> MGSDRSCVLSVFQTILKLVIFVAIFGAAISSRLFAVIKFESIIHEFDPWFNYRA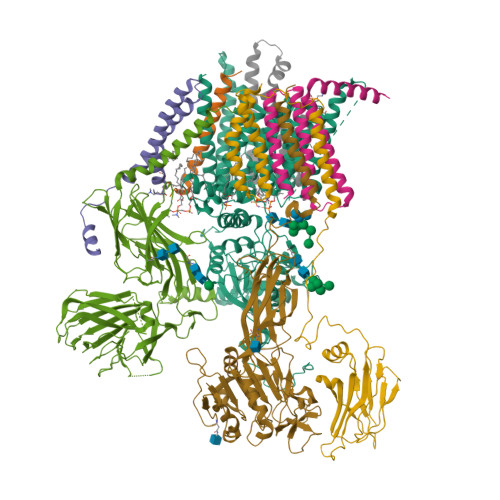TKYLVNNSFYKFLNWFDDRTWYPLGRVTGGTLYPGLMTTSAFIWHALRNWLGLPIDIRNVCVLFAPLFSGVTAWATYEFTKEIKDASAGLLAAGFIAIVPGYISRSVAGSYDNEAIAITLLMVTFMFWIKAQKTGSIMHATCAALFYFYMVSAWGGYVFITNLIPLHVFLLILMGRYSSKLYSAYTTWYAIGTVASMQIPFVGFLPIRSNDHMAALGVFGLIQIVAFGDFVKGQISTAKFKVIMMVSLFLILVLGVVGLSALTYMGLIAPWTGRFYSLWDTNYAKIHIPIIASVSEHQPVSWPAFFFDTHFLIWLFPAGVFLLFLDLKDEHVFVIAYSVLCSYFAGVMVRLMLTLTPVICVSAAVALSKIFDIYLDFKTSDRKYAIKPAALLAKLIVSGSFIFYLYLFVFHSTWVTRTAYSSPSVVLPSQTPDGKLALIDDFREAYYWLRMNSDEDSKVAAWWDYGYQIGGMADRTTLVDNNTWNNTHIAIVGKAMASPEEKSYEILKEHDVDYVLVIFGGLIGFGGDDINKFLWMIRISEGIWPEEIKERDFYTAEGEYRVDARASETMRNSLLYKMSYKDFPQLFNGGQATDRVRQQMITPLDVPPLDYFDEVFTSENWMVRIYQLKKDDAQGRTLRDVGELTRSSTKTRRSIKRPELGLRV;> MISDEQLNSLAITFGIVMMTLIVIYHAVDSTMSPKNRTLQVDGGSGGSLEVLFQGPTETSQVAPA;> MTYEQLYKEFHSSKSFQPFIHLDTQPKFAICGLIVTLAVLSSALFAVGSKSSYIKKLFFYTILSVIGSLFAGLTTVFASNSFGVYV;> MAKAPKANTPKVTSTSSAVLTDFQETFKTSKRAYFAQIEKYPKLKLIDTFCFFLVLLGVIQCTFIILIRDNFPFNAFLAGFIICVGQFVLLMSLRLQLCNSFPGISKNRAFAEFIVASLILHFVCLHFIN;> MRQVWFSWIVGLFLCFFNVSSAAQYEPPATWENVDYKRTIDVSNAYISETIEITIKNIASEPATEYFTAFESGIFSKVSFFSAYFTNEATFLNSQLLANSTTAPGDDGESEIRYGIIQFPNAISPQEEVSLVIKSFYNTVGIPYPEHVGMSEEQHLLWETNRLPLSAYDTKKASFTLIGSSSFEEYHPPNDESLLGKANGNSFEFGPWEDIPRFSSNETLAIVYSHNAPLNQVVNLRRDIWLSHWASTIQFEEYYELTNKAAKLSKGFSRLELMKQIQTQNMRQTHFVTVLDMLLPEGATDHYFTDLVGLVSTSHAERDHFFIRPRFPIFGGWNYNFTVGWTNKLSDFLHVSSGSDEKFVASIPILNGPPDTVYDNVELSVFLPEGAEIFDIDSPVPFTNVSIETQKSYFDLNKGHVKLTFSYRNLISQVANGQVLIKYDYPKSSFFKKPLSIACYIFTALMGVFVLKTLNMNVTN;> MQFFKTLAALVSCISFVLAYVAQDVHVSFPSTAGKSRVMIGKVEPRIGIDETVPTTITVEDPNEVIQVNFAIESTNKPFQNTLLIGLPNKNLEMAFEPEIKDNGKLSMYKYRIDLAKLDAALLQEASRSPEPIKATLILASSTAKPKENLFREILQLNLNFDVDHSDSSLVDKFGIKPEIHHIFHAEPKRVAKPIAVIFVLIIFITILSLIVTWLNSCAAAFNNIPTGVTAVYFLGFIATIVGFEVIFARYYLGTSIFETLFSSLYLGAPGLLTSTKFLRSFGTI;> MRTDWNFFFCILLQAIFVVGTQTSRTLVLYDQSTEPLEEYSVYLKDLEQRNYKLEYLDINSTSTTVDLYDKEQRLFDNIIVFPTKGGKNLARQIPVKQLIKFFENEGNILCMSSPGAVPNTIRLFLNELGIYPSPKGHVIRDYFSPSSEELVVSSNHLLNKYVYNARKSEDFVFGESSAALLENREQIVPILNAPRTSFTESKGKCNSWTSGSQGFLVVGFQNLNNARLVWIGSSDFLKNKNQDSNQEFAKELLKWTFNEKSVIKSVHAVHSHADGTSYDEEPYKIKDKVIYSVGFSEWNGEEWLPHIADDIQFELRQVDPYYRLTLSPSGNDSETQYYTTGEFILPDRHGVFTFLTDYRKIGLSFTTDKDVKAIRHLANDEYPRSWEISNSWVYISAICGVIVAWIFFVVSFVTTSSVGKKLETFKKTN;> MNWLFLVSLVFFCGVSTHPALAMSSNRLLKLANKSPKKIIPLKDSSFENILAPPHENAYIVALFTATAPEIGCSLCLELESEYDTIVASWFDDHPDAKSSNSDTSIFFTKVNLEDPSKTIPKAFQFFQLNNVPRLFIFKPNSPSILDHSVISISTDTGSERMKQIIQAIKQFSQVNDFSLHLPMDWTPIITSTIITFITVLLFKKQSKLMFSIISSRIIWATLSTFFIICMISAYMFNQIRNTQLAGVGPKGEVMYFLPNEFQHQFAIETQVMVLIYGTLAALVVVLVKGIQFLRSHLYPETKKAYFIDAILASFCALFIYVFFAALTTVFTIKSPAYPFPLLRLSAPFK> MFSAGHKIKGTVVLMPKNELEVNPDGSAVDNLNAFLGRSVSLQLISATKADAHGKGKVGKDTFLEGINTSLPTLGAGESAFNIHFEWDGSMGIPGAFYIKNYMQVEFFLKSLTLEAISNQGTIRFVCNSWVYNTKLYKSVRIFFANHTYVPSETPAPLVEYREEELKSLRGNGTGERKEYDRIYDYDVYNDLGNPDKSEKLARPVLGGS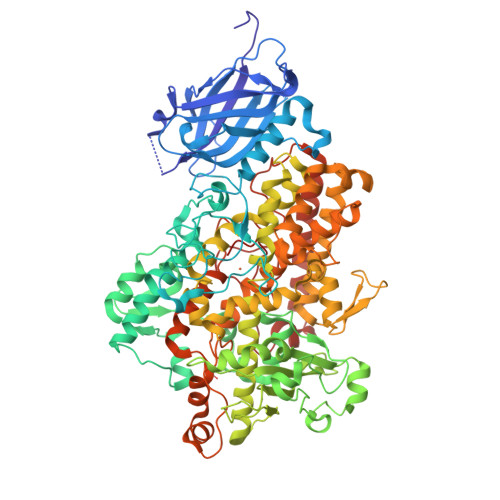STFPYPRRGRTGRGPTVTDPNTEKQGEVFYVPRDENLGHLKSKDALEIGTKSLSQIVQPAFESAFDLKSTPIEFHSFQDVHDLYEGGIKLPRDVISTIIPLPVIKELYRTDGQHILKFPQPHVVQVSQSAWMTDEEFAREMIAGVNPCVIRGLEEFPPKSNLDPAIYGDQSSKITADSLDLDGYTMDEALGSRRLFMLDYHDIFMPYVRQINQLNSAKTYATRTILFLREDGTLKPVAIELSLPHSAGDLSAAVSQVVLPAKEGVESTIWLLAKAYVIVNDSCYHQLMSHWLNTHAAMEPFVIATHRHLSVLHPIYKLLTPHYRNNMNINALARQSLINANGIGETTFLPSKYSVEMSSAVYKNWVFTDQALPADLIKRGVAIKDPSTPHGVRLLIEDYPYAADGLEIWAAIKTWVQEYVPLYYARDDDVKNDSELQHWWKEAVEKGHGDLKDKPWWPKLQTLEDLVEVCLIIIWIASALHAAVNFGQYPYGGLIMNRPTASRRLLPEKGTPEYEEMINNHEKAYLRTITSKLPTLISLSVIEILSTHASDEVYLGQRDNPHWTSDSKALQAFQKFGNKLKEIEEKLVRRNNDPSLQGNRLGPVQLPYTLLYPSSEEGLTFRGIPNSISI>[2x]GPLGSQELRLRVQGKEKHQMLEISLSPDSPLKVLMSHYEEAMGLSGHKLSFFFDG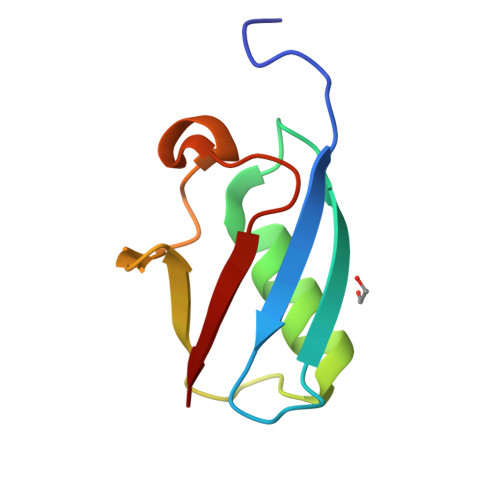TKLSGKELPADLGLESGDLIEVWG>[4x]MFSEELIKENENIWRRFLPH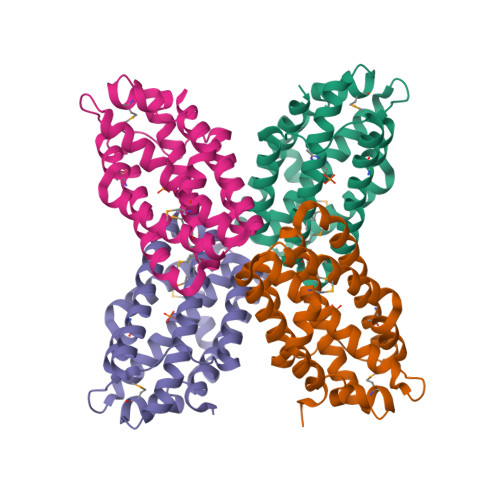KFLIEMAENTIKKENFEKWLVNDYYFVKNALRFMALLMAKAPDDLLPFFAESIYYISKELEMFEKKAQELGISLNGEIDWRAKSYVNYLLSVASLGSFLEGFTALYCEEKAYYEAWKWVRENLKERSPYQEFINHWSSQEFGEYVKRIEKILNSLAEKHGEFEKERAREVFKEVSKFELIFWDIAYGGEGNVLEHHHHHH>[2x]MASMAASATRHPYPFDRAVPTAIPPLYEELRETERVAAITMATGDPGFLVTRYEDVR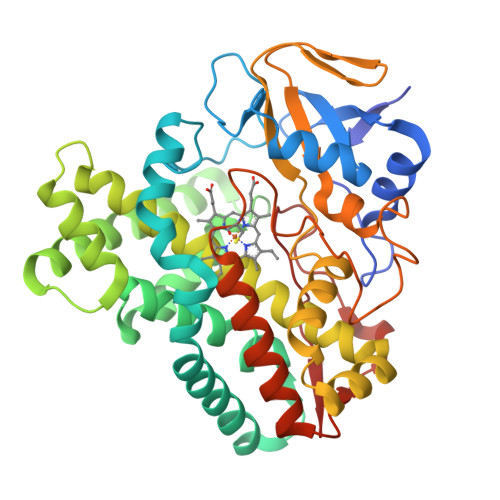FVLSDPRFSVRQDLPGAPRLTEMTFESVMTTDPPVHTRLRRLLSRDFTARRIERMRPRLEEIAEGLLDEMEKKGAPADIVESLAVPFPITVICELLGVPMVDVARFRGWADTMVSLTGYSMEDWTAARDALESYLDGLVAAKRENPGSDLLSALVATAAEDNELTDHDVRSLSLILLLAGYEPASNQLGSSVLTLLRFPDRLAELRRDPGLLPSAVEELMRYAPAGDGALFRVTLEDVTIGDTHIPANSAVLASTQAANWDPRRFDDPTGLRLDRPDNQHTALGHGIHFCLGAALARVELQVAIGALLRRFPRLALATDESGLRWSSPGSMLSGFAEIPVTW>[8x]MADEIQIGPGSATRLEFRRHFAATPEQLWAALTSPALLPAWLFARGWPMTECVFEPHKGGL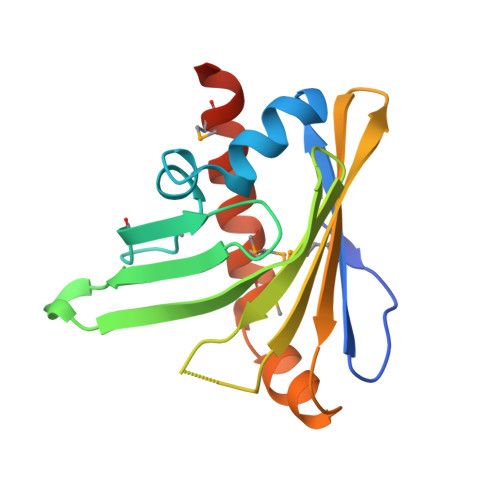IRQVWTGPEGRTRGLTGRVILAEPPHRLIHSELYDEDWTGGETLVTLQLLPVEGGTELAMAVDYATPEARDAVAASAMATEMEEAYRHLDVMLAALEHHHHHH> GVKIMPNLPGLYFLQAYPSEEIWRLFVDGRFWSKENGWRGYESREPGCLNAALESLCSIALQVEKSGEEFELSVDLIKRIHKKCGKKVEELQEKNPGELRTDEPVSFGIPAGRASIKGIEEFLSLVFLTEGGAEFGPGKAGPFGPRFDKNYFKNLNPEQIPDLAKQIYFDMCKYGHSNTNHFYLAVMKNVDVYLEKITQSYNKEIKTAETLDEKLKIIVKHIRMYEVLHPFRDANGRTFVNNLLNIPLMQQGLPPATFYEPNVFDLYSAEELVVVVKEAIFNTVEIIEQSKRKTPITLYGYHSSLEEQTKFRDMLDSPSYEKIKHMDFSDLNPEKLHLKTQKCLSSLNEQYPLHRGAIYLSDPGEIKLLLSNRNESQINQQIEQGAPPIYVGKTPAHLAVISGNMAMLDELIAKKAD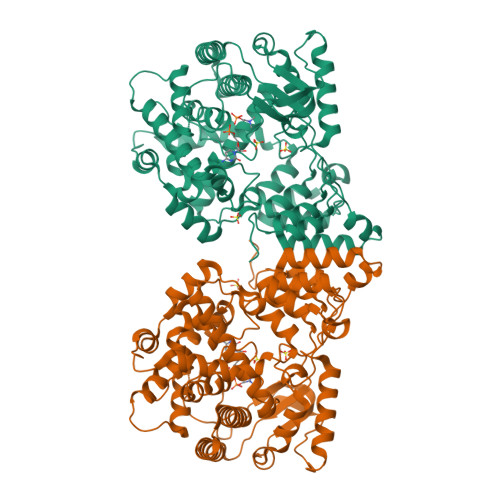LSLQDYDGKTALHYAAECGNMQIMGKILKVVLSQEDAIKVLNIKDNHGKTAFHYAAEFGTPELISAL N-{1-[5-chloro-3-methoxy-2-(1-methylethoxy)benzyl]piperidin-4-yl}-2-(2-methyl-4-sulfamoylphenoxy)acetamide 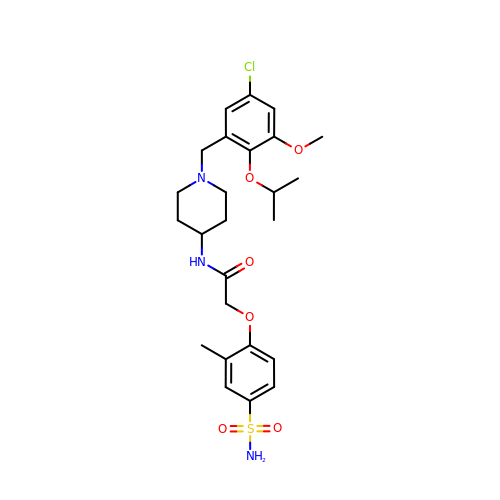| C25 H34 Cl N3 O6 S | IWMCULWPLNDDNK-UHFFFAOYSA-N(3S)-2,2-dimethyl-3-[(3E,7E,11E,15E)-3,7,12,16,20-pentamethylhenicosa-3,7,11,15,19-pentaen-1-yl]oxirane 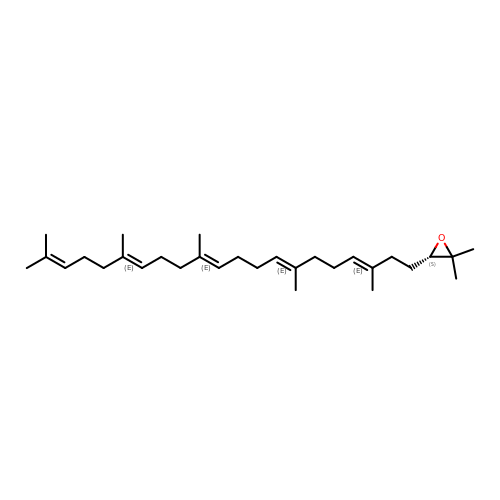| C30 H50 O | QYIMSPSDBYKPPY-RSKUXYSASA-N>[4x]MAEFRIAQDVVARENDRRASALKEDYEALGANLARRGVDIEAVTAKVEKFFVAVPSWGVGTGGTRFARFPGTGEPRGIFDKLDDCAVIQQLTRATPNVSLHIPWDKADPKELKARGDALGLGFDAMNSNTFSDAPGQAHSYKYGSLSH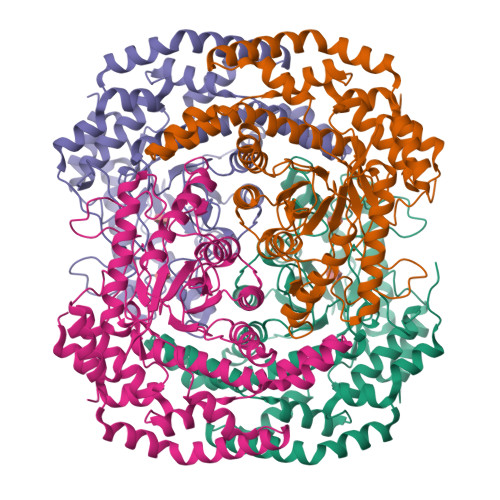TNAATRAQAVEHNLECIEIGKAIGSKALTVWIGDGSNFPGQSNFTRAFERYLSAMAEIYKGLPDDWKLFSEHKMYEPAFYSTVVQDWGTNYLIAQTLGPKAQCLVDLGHHAPNTNIEMIVARLIQFGKLGGFHFNDSKYGDDDLDAGAIEPYRLFLVFNELVDAEARGVKGFHPAHMINQSHNVTDPIESLINSANEIRRAYAQALLVDRAALSGYQEDNDALMATETLKRAYRTDVEPILAEARRRTGGAVDPVATYRASGYRARVAAERPASVAGGGGIIGSHHHHHH> GSHMTDLPRLPFDNPDIMGIAPQMLALQKEGPIARVGTAGEDAWLVTRYDEVRTLLADRRLRLSNPNPQPSAKSAARAFSVALMAGDDHETEPARHAQMRSLLIPRFSTRRLRLMKTRIEHHVDELLDQLAASAPPVDLHRVLSFRLPTMVVCDLLGVPLADRERFGQWARGTFDQSDNEHSANTFQQVVDYMLELVARKRVEPGDDILSELIAEKDGALSDADIAHLGNAVLLFGYETTIVRIDLGTLLLLRNPVQRAQLAEDPGLAPAAVEEILRLGVGGKGSNALIPRYAHGDITVGETVIRTGDAVMLAI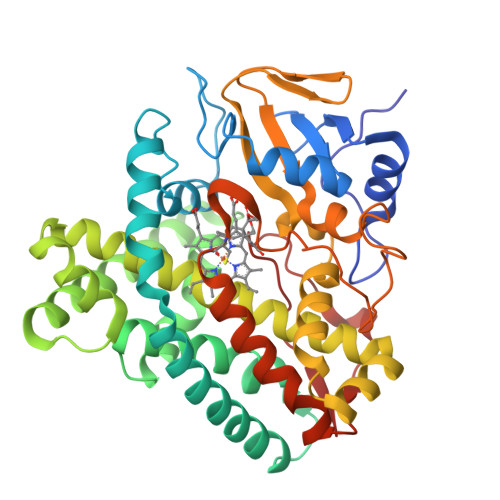GAANYDDRAFPDGGLFDLTRVRPRSHLAFGHGARHCIGRTLARIELTAVFERLFRRLPDLRLAVPEESLRWQEHRITGGFDEIPVTF>MDLRTMTQSLVTLAEDNIAFFSSQGPGETAQRLSGVFAGVREQALGLEPALGRLLGVAHLFDLDPETPANGYRSLVHTARCCLAHLLHKSRYVASNRRSIFFRTSHNLAELEAYLAALTQLRALVYYAQRLLVTNRPGVLFFEGDEGLTADFLREYVTLHKGCFYGRCLGFQFTPAIRPFLQTISIGLVSFGEHYKRNETGLSVAASSLFTSGRFAIDPELRGAEFERITQNLDVHFWKAFWNITEMEVLSSLANMASATVRVSRLLSLPPEAFEMPLTADPTLTVTISPPLAHTGPGPVLVRLISYDLREGQDSEELSSLIKSNGQRSLELWPRPQQAPRSRSLIVHFHGGGFVAQTSRSHEPYLKSWAQELGAPIISIDYSLAPEAPFPRALEECFFAYCWAIKHCALLGSTGERICLAGDSAGGNLCFTVALRAAAYGVRVPDGIMAAYPATMLQPAASPSRLLSLMDPLLPLSVLSKCVSAYAGAKTEDHSNSDQKALGMMGLVRRDTALLLRDFRLGASSWLNSFLELSGRKSQKMSEPIAEPMRRSVSEAALAQPQGPLGTDSLKNLTLRDLSLRGNSETSSDTPEMSLSAETLSPSTPSDVNFLLPPEDAGEEAEAKNELSPMDRGLGVRAAFPEGFHPRRSSQGATQMPLYSSPIV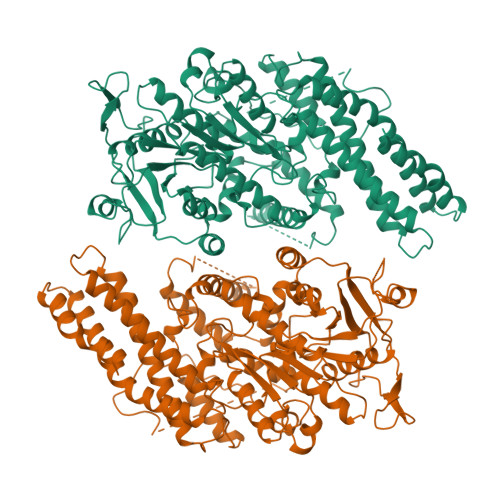KNPFMSPLLAPDSMLKSLPPVHIVACALDPMLDDSVMLARRLRNLGQPVTLRVVEDLPHGFLTLAALCRETRQAAELCVERIRLVLTPPAGAGPSGETGAAGVDGGCGGRH[2x]>[2x]MALADISGYLDVLDSVRGFSYL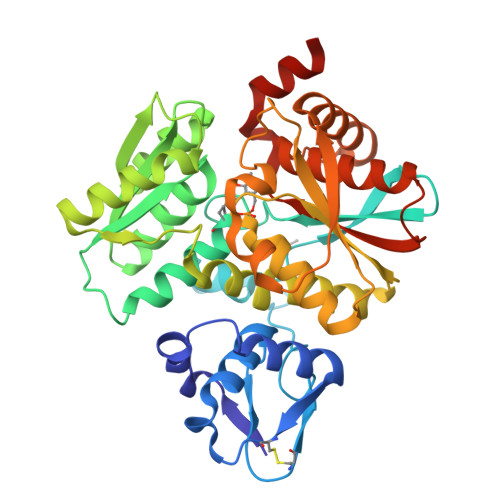ENAREVLRSGEARCLGNPRSEPEYVKALYVIGASRIPVGDGCSHTLEELGVFDISVPGEMVFPSPLDFFERGKPTPLVRSRLQLPNGVRVWLKLEWYNPFSLSVKDRPAVEIISRLSRRVEKGSLVADATSSNFGVALSAVARLYGYRARVYLPGAAEEFGKLLPRLLGAQVIVDPEAPSTVHLLPRVMKDSKNEGFVHVNQFYNDANFEAHMRGTAREIFVQSRRGGLALRGVAGSLGTSGHMSAAAFYLQSVDPSIRAVLVQPAQGDSIPGIRRVETGMLWINMLDISYTLAEVTLEEAMEAVVEVARSDGLVIGPSGGAAVKALAKKAAEGDLEPGDYVVVVPDTGFKYLSLVQNALEGAGDSV>[2x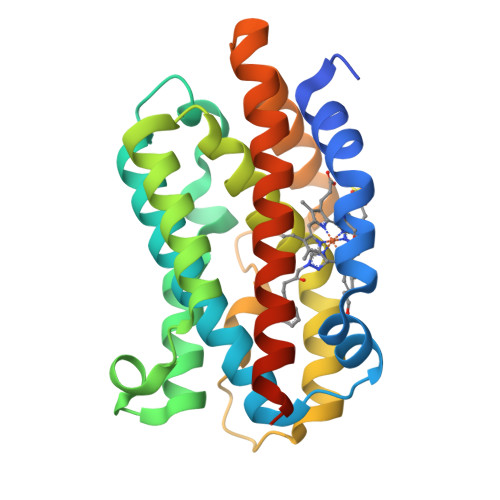]MERPQPDSMPQDLSEALKEATKEVHTQAENAEFMRNFQKGQVTRDGFKLVMASLYHIYVALEEEIERNKESPVFAPVYFPEELHRKAALEQDLAFWYGPRWQEVIPYTPAMQRYVKRLHEVGRTEPELLVAHAYTRYLGDLSGGQVLKKIAQKALDLPSSGEGLAFFTFPNIASATKFKQLYRSRMNSLEMTPAVRQRVIEEAKTAFLLNIQLFEELQELLTHDTKDQSPSRA5-[1-(ACETYLAMINO)-3-METHYLBUTYL]-2,5-ANHYDRO-3,4-DIDEOXY-4-(METHOXYCARBONYL)PENTONIC ACID | C14 H23 N O6 | 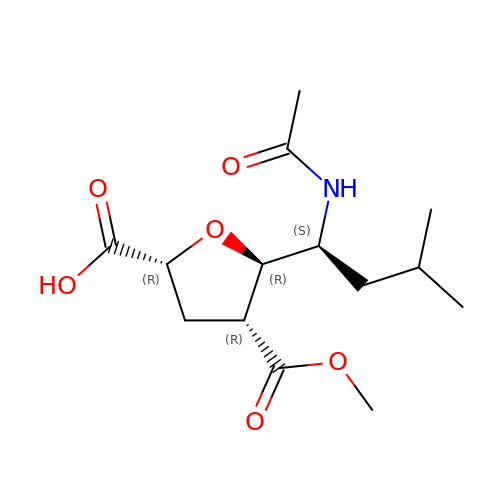MUJPWSPVNZGJOW-WRWGMCAJSA-N The proteins in the human epidermal growth factor receptor (HER or ErbB) family are some of the most thoroughly studied receptor tyrosine kinases. Ligand-induced homo- or hetero-dimerization of HER proteins initiates a downstream phosphorylation signaling cascade, which stimulates cell growth, proliferation, and differentiation. HER2 is unique within the HER family in that it does not have known ligands and cannot assemble into ligand-dependent homodimers. Thus, to facilitate downstream signaling, it must either form heterodimers with other HER proteins once their specific ligands have bound or self-assemble into ligand-independent homodimer under the condition of overexpression.

Finally, the complex structures of the EGF-bound EGFR/HER2 and homodimeric EGFR ectodomains were refined to 3.3 Å and 3.8 Å resolution, respectively. The EGFR–EGF/HER2 dimer adopted a heart-shaped structure, similar to the dimer structures of other family members. EGF wedged into the cleft between Domains I and III of EGFR, stabilizing it in the extended conformation and exposing the dimerization interface of Domain II. Accordingly, Domain II of EGFR resembled the canonical bent conformation seen in other dimer structures. On the other side of the complex, HER2 retained the same conformation as in its monomer form or in complex with HER3, consistent with its ligand-independent manner for signal transduction. Since Domain II of HER2 was presented in the unbent conformation, it dimerized with EGFR in an asymmetric manner, consistent with that of the NRG1β-bound HER2/HER3, EREG-bound human EGFR, and Spitz-bound Drosophila EGFR complexes. Specifically, for the EGFR/HER2 complex, both the N- and C-terminal regions of Domain II interacted more closely with their counterparts relative to the EGFR homodimer, burying 884 Å2 and 412 Å2 surface areas, respectively. Strikingly, the DAs of EGFR and HER2 adopted different conformations. The DA of HER2 was inserted properly into its binding pocket on EGFR and made extensive polar and nonpolar interactions, whereas the tip region of the EGFR DA was almost dissociated from HER2, maintaining little contact with Domain III. As a result, the total BSA between the DAs was only 1395 Å2 in the EGFR/HER2 complex (910 Å2 on the HER2 DA side and 485 Å2 on the EGFR DA side), which is less than that of the EGFR homodimer (1769 Å2).

> MRPSGTAGAALLALLAALCPASRALEEKKVCQGTSNKLTQLGTFEDHFLSLQRMFNNCEVVLGNLEITYVQRNYDLSFLKTIQEVAGYVLIALNTVERIPLENLQIIRGNMYYENSYALAVLSNYDANKTGLKELPMRNLQEILHGAVRFSNNPALCNVESIQWRDIVSSDFLSNMSMDFQNHLGSCQKCDPSCPNGSCWGAGEENCQKLTKIICAQQCSGRCRGKSPSDCCHNQCAAGCTGPRESDCLVCRKFRDEATCKDTCPPLMLYNPTTYQMDVNPEGKYSFGATCVKKCPRNYVVTDHGSCVRACGADSYEMEEDGVRKCKKCEGPCRKVCNGIGIGEFKDSLSINATNIKHFKNCTSISGDLHILPVAFRGDSFTHTPPLDPQELDILKTVKEITGFLLIQAWPENRTDLHAFENLEIIRGRTKQHGQFSLAVVSLNITSLGLRSLKEISDGDVIISGNKNLCYANTINWKKLFGTSGQKTKIISNRGENSCKATGQVCHALCSPEGCWGPEPRDCVSCRNVSRGRECVDKCNLLEGEPREFVENSECIQCHPECLPQAMNITCTGRGPDNCIQCAHYIDGPHCVKTCPAGVMGENNTLVWKYADAGHVCHLCHPNCTYGCTGPGLEGCPTNGPKIPSIATGMVGALLLLLVVALGIGLFMRRRHIVRKRTLRRLLGGSENLYFQGGGSAAQLKKKLQALKKKNAQLKWKLQALKKKLAQSNSLEVLFQ;> MELAALCRWGLLLALLPPGAASTQVCTGTDMKLRLPASPETHLDMLRHLYQGCQVVQGNLELTYLPTNASLSFLQDIQEVQGYVLIAHNQVRQVPLQRLRIVRGTQLFEDNYALAVLDNGDPLNNTTPVTGASPGGLRELQLRSLTEILKGGVLIQRNPQLCYQDTILWKDIFHKNNQLALTLIDTNRSRACHPCSPMCKGSRCWGESSEDCQSLTRTVCAGGCARCKGPLPTDCCHEQCAAGCTGPKHSDCLACLHFNHSGICELHCPALVTYNTDTFESMPNPEGRYTFGASCVTACPYNYLSTDVGSCTLVCPLHNQEVTAEDGTQRCEKCSKPCARVCYGLGMEHLREVRAVTSANIQEFAGCKKIFGSLAFLPESFDGDPASNTAPLQPEQLQVFETLEEITGYLYISAWPDSLPDLSVFQNLQVIRGRILHNGAYSLTLQGLGISWLGLRSLRELGSGLALIHHNTHLCFVHTVPWDQLFRNPHQALLHTANRPEDECVGEGLACHQLCARGHCWGPGPTQCVNCSQFLRGQECVEECRVLQGLPREYVNARHCLPCHPECQPQNGSVTCFGPEADQCVACAHYKDPPFCVARCPSGVKPDLSYMPIWKFPDEEGACQPCPINCTHSCVDLDDKGCPAEQRASPLTSIISAVVGILLVVVLGVVFGILIKRRQQKIRKYTMRRLLQEGGSENLYFQGGGSAQLEKELQALEKENAQLEWELQALEKELAQSNSLEVLFQ;> GPTANSDSECPLSHDGYCLHDGVCMYIEALDKYACNCVVGYIGERCQYRDLKWWELR[(2R,3S,4R,5R)-5-(2,4-DIOXO-3,4-DIHYDROPYRIMIDIN-1(2H)-YL)-3,4-DIHYDROXYTETRAHYDROFURAN-2-YL]METHYL (2R,3S,4R,5R)-5-(2,4-DIOXO-3,4-DIHYDROPYRIMIDIN-1(2H)-YL)-4-HYDROXY-2-(HYDROXYMETHYL)TETRAHYDROFURAN-3-YL 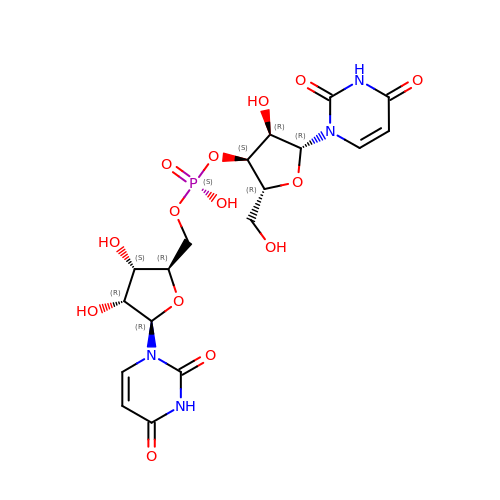HYDROGEN (S)-PHOSPHATE | C18 H23 N4 O14 P | KXSPLNAXPMVUEC-NCOIDOBVSA-N>MTMDEQQSQAVAPVYVGGFLARYDQSPDEAELLLPRDVVEHWLHAQGQGQPSLSVALP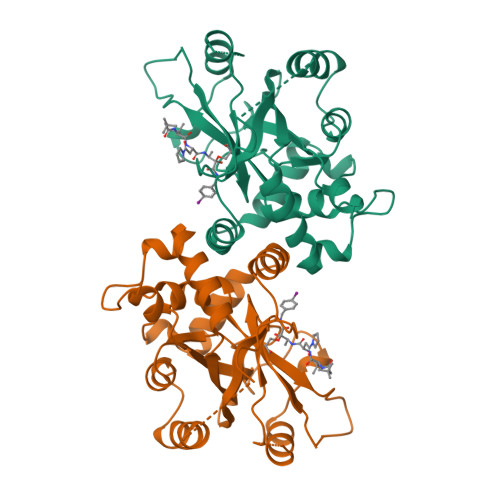LNINHDDTAVVGHVAAMQSVRDGLFCLGCVTSPRFLEIVRRASEKSELVSRGPVSPLQPDKVVEFLSGSYAGLSLSSRRCDDVEQATSLSGSETTPFKHVALCSVGRRRGTLAVYGRDPEWVMQRFPDLTAADRDGLRAQWQRCGSTAVDASGDPFRSDSYGLLGNSVDAMYIRERLPKLRYDKQLVGVTERESYVKA[4x]>[2x]GSGRTEIDKPSQMQVTDVQDNSISVKWLPSSSPVTGYRVTTTPKNGPGPTKTKTAGPDQTEMTIEGLQPTVEYVVSVYAQNPSGESQPLVQTAVTNIDRPKGLAFTDVDVDSIKIAWESPQGQVSRYRVTYSSPEDGIHELFPAPDGEEDTAELQGLRPGSEYTVSVVALHDDMESQ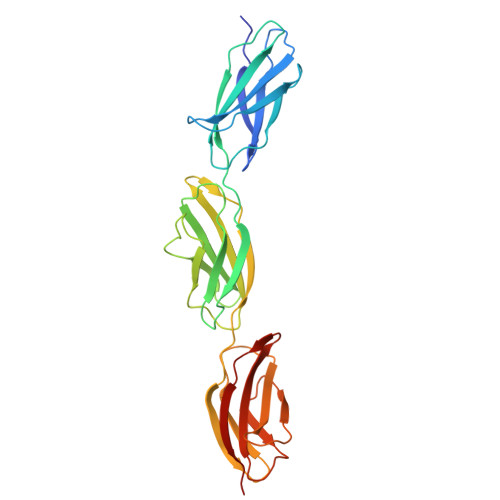PLIGTQSTAIPAPTDLKFTQVTPTSLSAQWTPPNVQLTGYRVRVTPKEKTGPMKEINLAPDSSSVVVSGLMVATKYEVSVYALKDTLTSRPAQGVVTTLE> SNILEMKELIVYFSTQSNNTHRFVQKLDAESIRIPIDEEERIKVDEDYVLIVPTYSGGKVTDAGQVDAHGAVPKQVIHFLNDPDNRKHCLGVISSGNTNFGDSFAIAGPVISYKLKVPLLYQFELIGTKEDVEEVNRIISETFN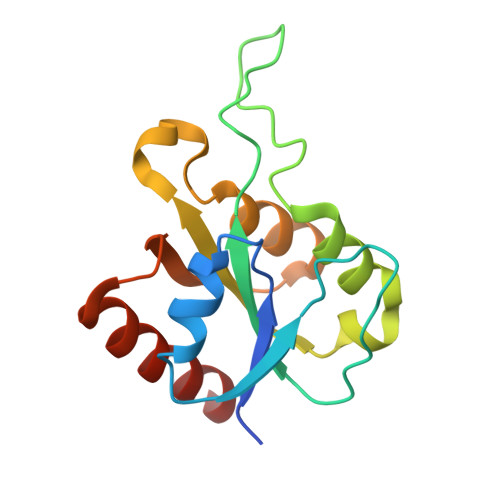ADQ>[12x]MIDDLFAGLPALEKGSVWLVGAGPGDPGLLTLHAANALRQADVIVHDALVNEDCLKLARPGAVLEFAGKRGGKPSPKQRDISLRLVELARAGNRV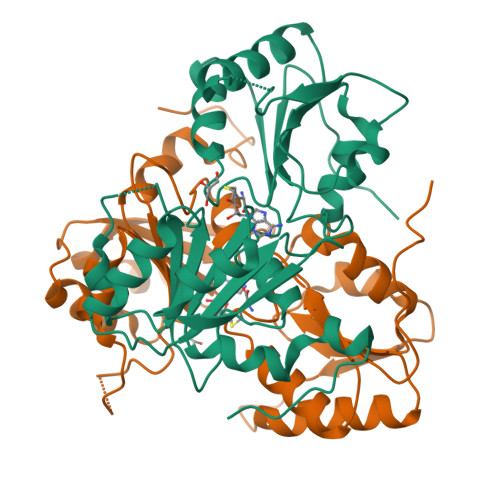LRLKGGDPFVFGRGGEEALTLVEHQVPFRIVPGITAGIGGLAYAGIPVTHREVNHAVTFLTGHDSSGLVPDRINWQGIASGSPVIVMYMAMKHIGAITANLIAGGRSPDEPVAFVCNAATPQQAVLETTLARAEADVAAAGLEPPAIVVVGEVVRLRAALDWIGALDGRKLAADPFANRILRNPA1-[4-[[(2~{E})-2-(4-chloranylcyclohexa-2,4-dien-1-ylidene)-1,3-dihydroimidazol-4-yl]carbonyl]piperazin-1-yl]-2,2-dimethyl-propan-1-one 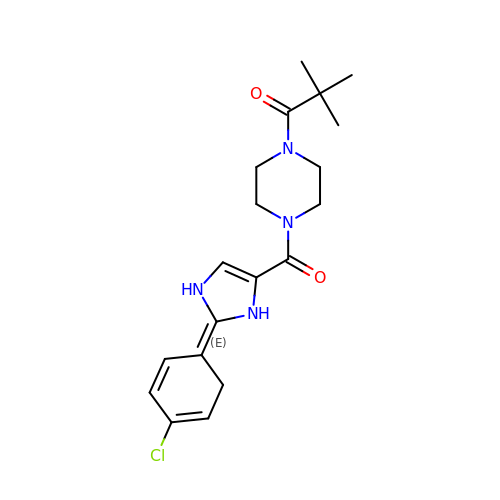| C19 H25 Cl N4 O2 | NKIIVXBCLGCNED-SSZFMOIBSA-N> MYGIQTSASLPLTRPQALETQAAAPQSDAPDASAGQTRAAPQGSAAPALAAARAKADELGQAAREVRASVERQTAYETRLAAQRSAAAFSGGEPPQARREAPGAELDEARNAQTVSARLFEGNLKGVAQSGHAMSAEQKQALQSGLDDVFADAPPQARSAGAPMLYSANAAAGQGMADSDLWDMISDQIGKIKDNYLGVYENVVGQYTDFYKAFSDILSQMANWIKPGGDGNKVKLNVDALKAALEKLKKDFSLGDNLDNKKAVLFPAQSKDGGIQGGSESDARKWAKEMGLPDAPPPGFSCVQKAADGNWVVVVDMTPIDTMIRDVGALGSGTELELDNAKFQAWQSGFKAQEENLKNTLQTL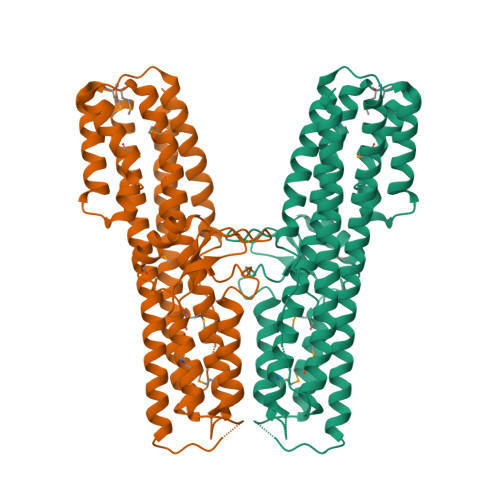TQKYSNANSLFDNLVKVLSSTISSCLETAKSFLQILEHHHHHH(2R,4S,5S)-N-[(2S,3R,4S)-1-cyclohexyl-3,4-dihydroxy-6-methylheptan-2-yl]-2-(cyclopropylmethyl)-4,5-dihydroxy-6-phenylhexanamide 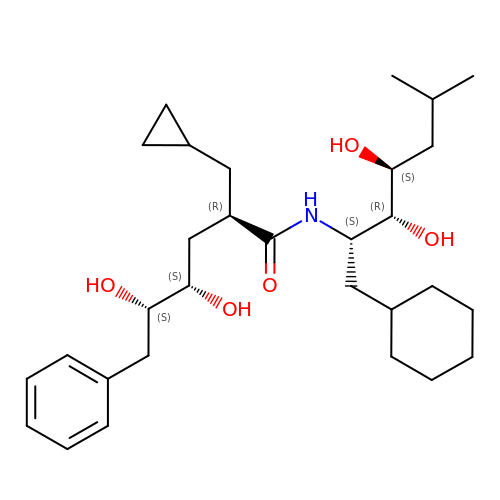| C30 H49 N O5 | LRMIUNSMKAGCAH-ZGLCPUQGSA-N The anaphase-promoting complex/cyclosome (APC/C) is a large multimeric cullin-RING E3 ubiquitin ligase that functions to regulate cell cycle transitions by ubiquitinating specific cell cycle regulatory proteins and targeting them for proteolysis by the ubiquitin-proteasome system. Only four subunits are directly involved in catalyzing protein ubiquitination (the cullin subunit Apc2 and the RING subunit Apc11) and degron recognition [coactivator subunits (either Cdc20 or Cdh1) and Apc10]. The remaining 85% of the APC/C mass corresponds to scaffolding subunits, of which seven are large multiple repeat motif proteins (Apc1 and Apc3–Apc8). Seeking to obtain insights into these structures at atomic resolution and to assist in the interpretation of cryo-EM reconstructions of the APC/C complex, we determined the crystal structures of full-length Apc4 and the N-terminal domain of Apc5 (Apc5N).

We purified residues 1–161 of X. laevis Apc5 as a bi-product of the Apc4–Apc5N coexpression system and crystallized the protein. The structure was determined to 2.2 Å resolution using single-wavelength anomalous diffraction phasing. Apc5N [residues 27–161 (human Apc5 numbering)] adopts an all α-helical domain architecture comprising seven α-helices. Helices α1–α6 pack to create an antiparallel bundle with α1 at the center of the domain almost completely surrounded by helices α2–α6. This α-helical domain is capped by α7, orientated orthogonally to the α-helical domain. In the crystal structure, residues 164–168 from the TEV cleavage site continue the α7 helix, similar in structure to α7 of human Apc5N defined in the EM density map. Residues 1–26 of Apc5N, predicted to form two α-helices, are disordered in both the crystal structure and the EM density map. A small shift of the loop connecting α5 with α6 accommodates the Apc4–Apc5 interface within the context of the APC/C. A larger 6-Å-conformational change involving the loop connecting α1 with α2 and the N-terminus of α2 results from both packing at the Apc4–Apc5 interface and a two-residue insertion within human Apc5 relative to X. laevis Apc5. DALI searches revealed weak structural similarity to the RNP assembly factor, although the biological significance of this similarity is unclear.

> MASVHESLYFNPMMTNGVVHANVFGIKDWVTPYKISVLVLLSEMSKNTKISLVEKRRLNKQILPLLQGPDMTLSKLIKIVEECCPNVSSSVHIRIKLMAEGELKDMEQFFDDLADSFTGTEPEVHKTSVVGLFLRHMILAYNKLSFSQVYKLYTSLQQYFQSDENLYFQ> MANETQTQKSTGVANDASLSLLDEILSEAKLKPKDEGYDVAKRGVQAFITEMLAPNRSEERVDKALVDAMIAEIDKRLSSQVNEILHAKEFQKLESSWRSLKFMVDRTDFRENTRVEMLNASKEDLQKDFEDAPEVTKSGLYKLVYSNEYGVFGGKPYGIISANYDFNVGPQDMELLRKCASVAAMAHAPFIGNAAPEVFGEESFLKLPDLKDLKSLFE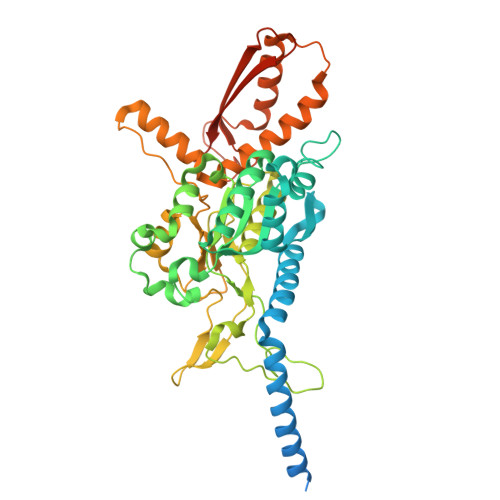GPQYARWHSFRESEDARYVGLALPRFLLRLPYGEKTVPVKAFNFTEDVVGHHERYLWGHASVALTSRVADSFAKFRWSPNIIGPQSGGAVENLPLHQYEAMGEIQTKIPTEVMLTERREFELSEEGFIGLVFRKDSDNAAFFSANSTQKPRFFGNTPEGKAAETNYRLGTQLPYMFIMTRLAHYIKVLQREQIGSWKEKSDLERELNHWLSQYISDMDDPAPAVRSRRPLRAARVVVEDVEGQPGWYRCSLQVRPHFKYMGASFTLSLVGKLDKE> MDETGKELVLALYDYQEKSPDEVTMKKGD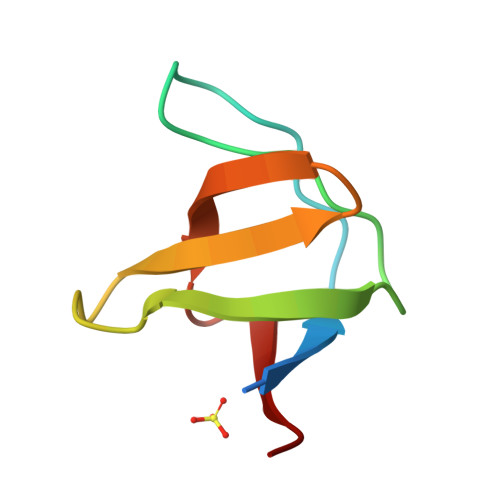ILTLLNSTNKDWWKVEVNDRQGFVPAAYVKKLD>[235x]MAQQSTKNETALLVAKSAKSALQDFNHDYSKSWTFGDKWDNSNTMFETFVNKYLFPKINETLLIDIALGNRFNWLAKEQDFIGQYSEEYVIMDTVPINMDLSKNEELMLKRNYPRMATKLYGNGIVKKQKFTLNNNDTRFNFQTLADATNYALGVYKKKISDINVLEEKEMRAMLVDYSLNQLSETNVRKATSKEDLASKVFEAILNLQNNSAKYNEVHRASGGAIGQYTTVSKLKDIVILTTDSLKSYLLDTKIANTFQIAGIDFTDHVISFDDLGGVFKVTKEFKLQNQDSIDFLRAYGDYQSQLGDTIPVGAVFTYDVSKLKEFTGNVEEIKPKSDLYAFILDINSIKYKRYTKGMLKPPFHNPEFDEVTHWIHYYSFKAISPFFNKILITDQDVNPKPEEELQE;>[12x]MNNDKRGLNVELSKEISKRVVEHRNRFKRLMFNRYLEFLPLLINYTNRDTVGIDFIQLESALRQNINVVVGEARNK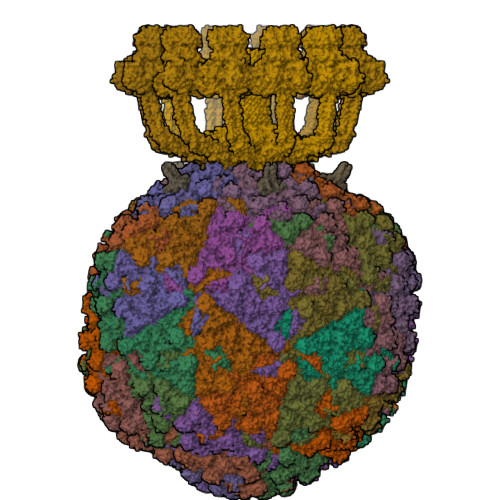QIMILGYVNNTYFNQAPNFSSNFNFQFQKRLTKEDIYFIVPDYLIPDDCLQIHKLYDNCMSGNFVVMQNKPIQYNSDIEIIEHYTDELAEVALSRFSLIMQAKFSKIFKSEINDESINQLVSEIYNGAPFVKMSPMFNADDDIIDLTSNSVIPALTEMKREYQNKISELSNYLGINSLAVDKESGVSDEEAKSNRGFTTSNSNIYLKGREPITFLSKRYGLDIKPYYDDETTSKISMVDTLFKDESSDING;>MARYTMTLYDFIKSELIKKGFNEFVNDNKLTFYDDEFQFMQKMLKFDKDVLAIVNEKVFKGFSLKDELSDLLFKKSFTIHFLDREINRQTVEAFGMQVITVCITHEDYLNVVYSSSEVEKYLQSQGFTEHNEDTTSNTDETSNQNATSLDNSTGMTANRNAYVSLPQSEVNIDVDNTTLRFADNNTIDNGKTVNKSSNESNQNAKRNQNQKGNAKGTQFTKQYLIDNIDKAYDLRKKILNEFDKKCFLQIW[12x];>MAYNENDFKYFDDIRPFLDEIYKTRERYTPFYDDRADYNTNSKSYYDYISRLSKLIEVLARRIWDYDNELKKRFKNWDDLMKAFPEQAKDLFRGWLNDGTIDSIIHDEFKKYSAGLTSAFALFKVTEMKQMNDFKSEVKDLIKDIDRFVNGFELNELEPKFVMGFGGIRNAVNQSINIDKETNHMYSTQSDSQKPEGFWINKLTPSGDLISSMRIVQGGHGTTIGLERQSNGEMKIWLHHDGVAKLLQVAYKDNYVLDLEEAKGLTDYTPQSLLNKHTFTPLIDEANDKLILRFGDGTIQVRSRADVKNHIDNVEKEMTIDNSENNDNRWMQGIAVDGDDLYWLSGNSSVNSHVQIGKYSLTTGQKIYDYPFKLSYQDGINFPRDNFKEPEGICIYTNPKTKRKSLLLAMTNGGGGKRFHNLYGFFQLGEYEHFEALRARGSQNYKLTKDDGRALSIPDHIDDLNDLTQAGFYYIDGGTAEKLKNMPMNGSKRIIDAGCFINVYPTTQTLGTVQELTRFSTGRKMVKMVRGMTLDVFTLKWDYGLWTTIKTDAPYQEYLEASQYNNWIAYVTTAGEYYITGNQMELFRDAPEEIKKVGAWLRVSSGNAVGEVRQTLEANISEYKEFFSNVNAETKHREYGWVAKHQK[72x];>[235x]MYEGNNMRSMMGTSYEDSRLNKRTELNENMSIDTNKSEDSYGVQIHSLSKQSFTGDVEEE;>[72x]MTEFDEIVKPDDKEETSESTEENLESTEETSESTEESTEESTEESTEDKTVETIEEENENKLEPTTTDEDSSKFDPVVLEQRIASLEQQVTTFLSSQMQQPQQVQQTQSDVTESNKEDNDYSDEELVDKLDLD;>[15x]AAAAAAAAAAAAAAAAAAAAAAAAAAAAAAAAAAAAAAAAAAAAAAAAAAAAAAA;>AAAAAAAAAAAAAAAAA[15x]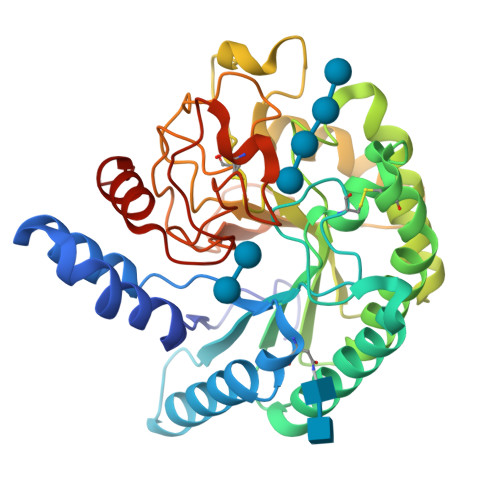> TASYNGNPFSGVQLWANTYYSSEVHTLAIPSLSPELAAKAAKVAEVPSFQWLDRNVTVDTLFSGTLAEIRAANQRGANPPYAGIFVVYDLPDRDCAAAASNGEWSIANNGANNYKRYIDRIRELLIQYSDIRTILVIEPDSLANMVTNMNVQKCSNAASTYKELTVYALKQLNLPHVAMYMDAGHAGWLGWPANIQPAAELFAQIYRDAGRPAAVRGLATNVANYNAWSIASPPSYTSPNPNYDEKHYIEAFAPLLRNQGFDAKFIVDTGRNGKQPTGQLEWGHWCNVKGTGFGVRPTANTGHELVDAFVWVKPGGESDGTSDTSAARYDYHCGLSDALTPAPEAGQWFQAYFEQLLINANPPF> MTAVVKNLAKLPAATSQILTNVSKLQTFHGLLEERRDKYAPLAYHTYDNLKQKTTWHPIAHAWVDEGLPVSKKEYNEYCWLKKDMQRLLPLASPFVFGIYGILPLAVWLSNDGYLPSAFSSKKDIVSKKLEWYSSY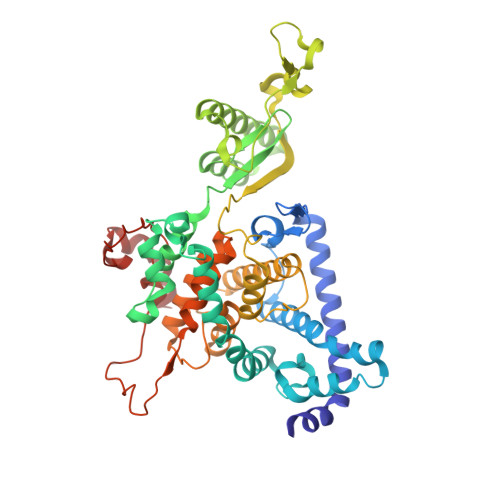GDDLRQQVGPMLQHRLKRHLRGTLNNEHRLMLDEVTESYKEIFYSHYTGQLRDVRKCAHLRLYDGTSTVLLLTNKEPVELTSELLQKWNAIKAAKLSPEEEKKARNEALIEAYKEQELHGGPHVKHMQGYGIPADTPLLGENAKGDQYTQPPESASIPLEQLEWTGDTVFIPAEYRTEMEDWGRELTKLANQFLLLPWRFVSNAWNQRRLVSWFEEILQEDALIAKEGGVQALSDDELKVALLDRAVIRCDEELTRGDMEARYKEISWLMSLRNPFIVLAWQTGYYRSTYSPEDDLPEASILPKLNRTVLDVDVHNELAPDHPEKPLPRVHPALYPNSHLALAKEVAVLAK>MQFRSIIRIVGLLLALFSVTMLAPALVALLYRDGAGVPFVTTFFVLLFCGAMCWFPNRRHKHELKSRDGFLIVVLFWTVLGSAGSLPFLIADNPNISVTDAFFESFSALTTTGATVIVGLDELPKAILFYRQFLQWFGGMGIIVLAVAILPVLGIGGMQLYRAEIPGPVKDTKMTPRIAETAKALWYIYLSLTIACAVAFWLAGMTPFDAISHSFSTIAIGGFSTHDASMGYFDSYAINLITVVFLLISACNFTLHFAAFASGGVHPKYYWKDPEFRAFIFIQVLLFLVCFLLLLKHHSYTSPYDAFDQALFQTVSISTTAGFTTTGFADWPLFLPVLLLFSSFIGGCAGSTGGGMKVIRILLLTLQGARELKRLVHPRAVYTIKVGGSALPQRVVDAVWGFFSAYALVFVVCMLGLIATGMDELSAFSAVAATLNNLGPGLGEVALHFGDVNDKAKWVLIVSMLFGRLEIFTLLILLTPTFWRS[2x];>[2x]MKIIILGAGQVGGTLAENLVGENNDITIVDNNADRLRELQDKYDLRVVNGHASHPDVLHEAGAQDADMLVAVTNTDETNMAACQVAFTLFNTPNRVARIRSPEYLAEKEALFKSGAIPVDHLIAPEELVTSYIERLIQYPGALQVVSFAEQKVSLVAVKAYYGGPLVGNALSALREHMPHIDTRVAAIFRQGRPIRPQGTTIIEADDEVFFVAASNHIRSVMSELQRLEKPYRRIMIVGGGNIGASLAKRLEQTYSVKLIERDYQRAEKLSEQLENTIVFCGDAADQELLTEENIDQVDVFIALTNEDETNIMSAML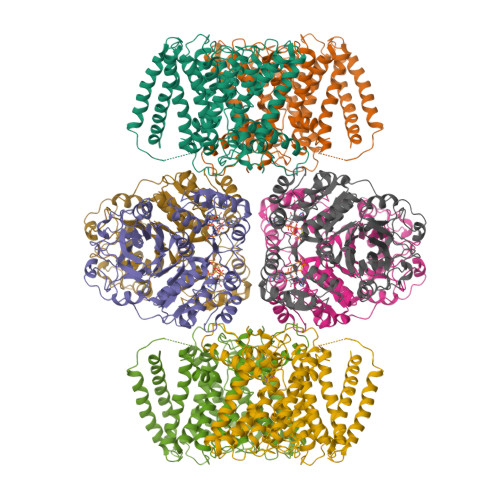AKRMGAKKVMVLIQRGAYVDLVQGGVIDVAISPQQATISALLTHVRRADIVNVSSLRRGAAEAIEAVAHGDETTSKVVGRAIGDIKLPPGTTIGAVVRGEEVLIAHDRTVIEQDDHVVMFLVDKKYVPDVEALFQPSPFFL>[2x]MKFTVEREHLLKPLQQVSGPLGGRPTLPILGNLLLQVADGTLSLTGTDLEMEMVARVALVQPHEPGATTVPARKFFDICRGLPEGAEIAVQLEGERMLVRSGRSRFSLSTLPAADFP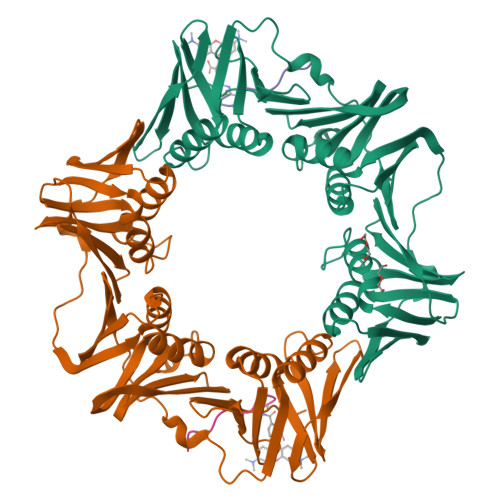NLDDWQSEVEFTLPQATMKRLIEATQFSMAHQDVRYYLNGMLFETEGEELRTVATDGHRLAVCSMPIGQSLPSHSVIVPRKGVIELMRMLDGGDNPLRVQIGSNNIRAHVGDFIFTSKLVDGRFPDYRRVLPKNPDKHLEAGCDLLKQAFARAAILSNEKFRGVRLYVSENQLKITANNPEQEEAEEILDVTYSGAEMEIGFNVSYVLDVLNALKCENVRMMLTDSVSSVQIEDAASQSAAYVVMPMRL;>[2x]SEQVELEFD> CTVPIGWSEPVKGLCKARFTRYYCMGNCCKVYEGCYTGGYSRMGECAR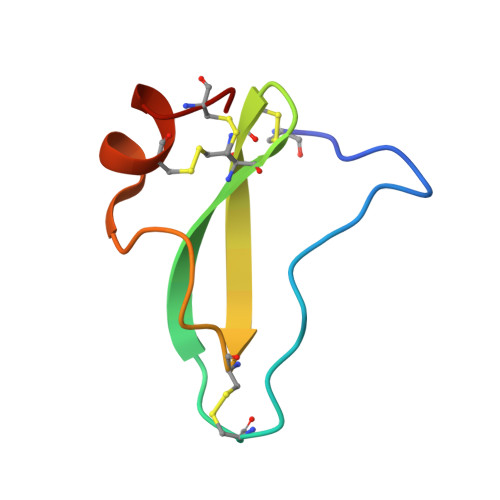NCPA> MIKPMRIFIGGEELETYTSARLQRTKKQLTGSLTVEIFLNYVPSKPVIVNAVRGKEILVYVMGELAFTGIIDKRKGKTVAGSQPRDASGRFAYSGGPGSMSDEGGSDVTVNFAKGQGYSVTLTARGRTKYLVDSSHSHPTGSFKDTSDRKVIEALVKEHKVVLDWQGTEVKEPKITLRDGNRIFNEIFERCNQNCHFAYETRDGKLLVTDGTTGVVGEDIVLGQNILDFSAEQSEDRANSEITVKGHRVAKDVWGKNAIVQPVQSVADSWVGANIPLTIQHYGDATNESLQRRAKFEADRRAAESKSVNVTVFHVAQQGGIPWDIGNIHYVEIPPEGIFDVMECVSLTYSV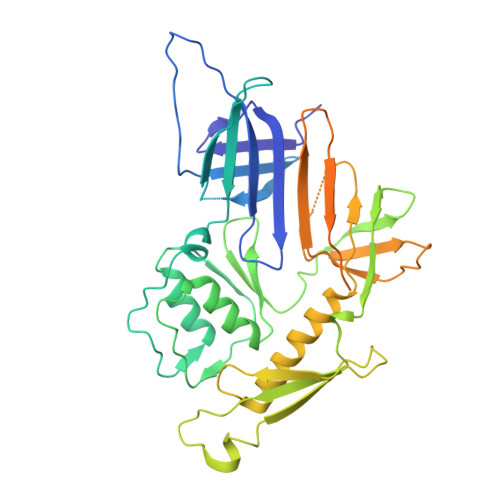DAKSTLETQLELAPPPSESISGASSGLLSSISNSLADISTKGVARRVQAGIKLIAGQYPSTWTSAALSAITTPVNVIASVVNSLLLNEDESTPKQPPLRLPPE> MLARKSIIPEEYVLARIAAENLRKPRIRDRLPKARFIAKSGACNLAHKNIREQGRFLQDIFTTLVDLKWRHTLVIFTMSFLCSWLLFAIMWWLVAFAHGDIYAYMEKGITEKSGLESAVCVTNVRSFTSAFLFSIEVQVTIGFGGRMMTEECPLAITVLILQNIVGLIINAVMLGCIFMKTAQAHRRAETLIFSRHAVIAVRNGKLCFMFRVGDLRKSMIISASVRIQVVKKTTTP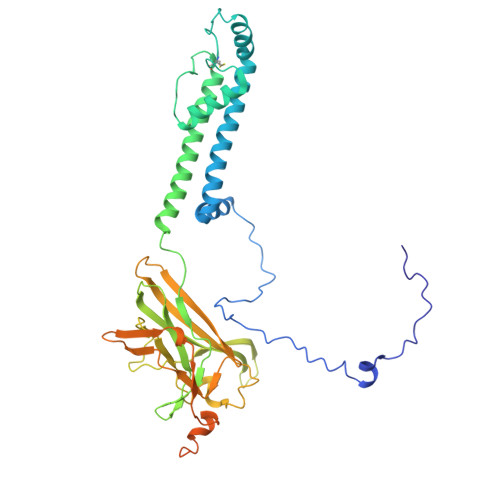EGEVVPIHQQDIPVDNPIESNNIFLVAPLIICHVIDKRSPLYDISATDLVNQDLEVIVILEGVVETTGITTQARTSYIAEEIQWGHRFVSIVTEEEGVYSVDYSKFGNTVRVAAPRCSARELDEKPSILIQTLQKSELSHQNSLRKRNSMRRNNSMRRSNSIRRNNSSLMVPKVQFMTPEGNQCPSES While this crucial step in protein maturation is executed by two types of methionine aminopeptidases in eukaryotes (MAP1 and MAP2), additional roles in disease and translational regulation have drawn more attention to MAP2. While MAP1 and MAP2 share the common pita-bread fold, the latter is additionally characterized by the presence of several insertions and a charged N-terminal extension, which consists of segmented regions of alternating poly-acidic and poly-basic stretches. However, the major determinant for binding to the tunnel exit is the MAP2-specific insert domain of ~60 residues, which is locked in between uL23, the universal binding site for nascent chain associated factors, eL19, and 28S rRNA helices H53 and H59 (also termed ES24L). Taken together, our data show that it is the insert domain that specifically directs MAP2 to the site of action on the 80S ribosome, either the PTE or the A-site.

In order to build CtMAP2 into the cryo-EM density, the crystal structure of CtMAP2(∆N2-73) was solved at 1.3 Å resolution. In combination, these tools allowed for a detailed structural analysis of MAP2 bound to the ribosome.

> PGSGSPTQQSDPPRVLISHLFPDGKYPAGEEVEYVNENRYRTTSEEKRYLDNMQSEFLNDYRQAAEVHRQVRKWAQGFVKPGKSLIEISEGIEDSVRALVGHPGLEEGDALKAGMGFPVGLSINHCAAHYNPNSGNKIVLQQDDVIKIDIGVHVNGRIVDSAFTMAWNDQFNPLLEAVRAATNAGIREAGIDARVGEIGGVIQEVMESYEVEINGKTYPVKPIRNLNGHNILPYSIHGTKSVPIVKTHDQTKMEEGDVFAIETFGSTGKGYVIESGEVSHYALRGDAPKVDLRLSSAKSLLNVIKRHFGTLPFCRRFLDRLGQEKYLLGLNNLVSNGIVEDYPPLVDEKGSYTAQFEHTILIRPTVKEVISRGDDY>MISQFNQPRGSTSIEVNKQSIARNFGVKEDEVIYFTAGIDLSGFKVIYDESTQRAYSLPFGIVSGTTAISLDERAILTHSAGSVDLGELAVSREEYVTLPGSFNFGHTINVKNELLVHDDKKYRWDGSLPKVVAAGSTPDSSGGVGLGAWLSVGDAALRAELNTKVSDGTFPATIKYKYGLPSVIDGAIYRTVQDKLDDFVFLEDFGGKDDAGSTDNSIAFRKAFASGARKIRLRGSGVYGMATRDIELPAKYEIIGNAKNPEIKYLGTDTSFTMFTLTGSGPASNQWKQGGMFRDLIISSDVKINWMLGRHVQNLDYDRVFFYNSATVLNNYHYVNFTRCERWGSAFIGRADLNTIQFISESPKFHLCFSSGSPIDVWDTADLAITKCTMFAGDYAVRTRVTQKQVTAPDLFAGYPVLITCSVFDAVRGHAWDLEGSVYSTITGNLVSAGRDTNSHGAYIKGGRSLSLTGNVFTYCGNY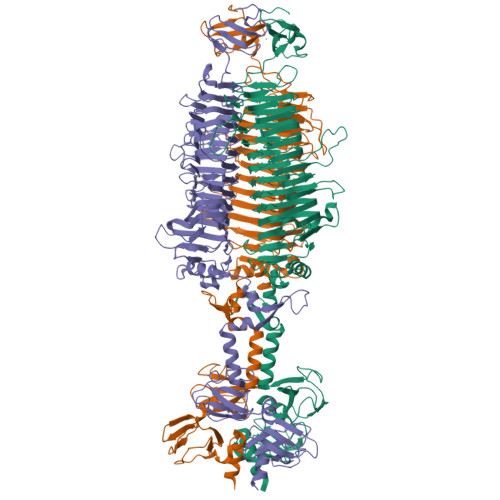GLVLEDVQQSGFVGNVFNGNKTGGLGTLACKDLSIVGGSMGTTYVRGGYYTQPVGYSDISSNSTGILLSGVAFDEALTTKVYLDTSITTRNKVINCSGVPDTIARGSTANRPANPQASYQYYDTTLGIPIWWNSVSGTWKNAAGADVLEHHHHHH[3x]>SELFIVRQLLQIVKQKTNQNSVDTTLKFTLSALWNLTDESPTTCRHFIENQGLELFMRVL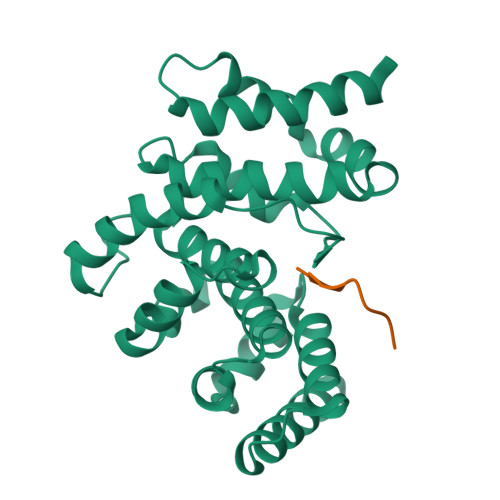ESFPTESSIQQKVLGLLNNIAEVQELHSELMWKDFIDHISSLLHSVEVEVSYFAAGIIAHLISRGEQAWTLSRSQRNSLLDDLHSAILKWPTPECEMVAYRSFNPFFPLLGCFTTPGVQLWAVWAMQHVCSKNPSRYCSMLIEEGGLQHLYNIKDHEHTDPHVQQIAVAILDSLEKHIVR[4x];>GYINVFA[4x]> NSSTASKTYNYVYSSDPSSLNYLAENRAATSDIVANLVDGLLENDQYGNIIPSLAEDWTVSQDGLTYTYKLRKDAKWFTSEGEEYAPVTAQDFVTGLQYAADKKSEALYLVQDSVAGLDDYITGKTSDFSTVGVKALDDQTVQYTLVKPELYWNSKTLATILFPVNADFLKSKGDDFGKADPSSILYNGPFLMKALVSKSAIEYKKNPNYWDAKNVFVDDVKLTYYDGSDQESLERNFTAGAYTTARLFPNSSSYEGIKEKYKNNIIYSMQNSTSYFFNFNLDRKSYNYTSKTSDIEKKSTQEAVLNKNFRQAINFAFDRTSYGAQSEGKEGATKILRNLVVPPNFVSIKGKDFGEVVASKMVNYGKEWQGINFADGQDPYYNPEKAKAKFAEAKKELEAKGVQFPIHLDKTVEVTDKVGIQGVSSIKQSIESVLGSDNVVIDIQQLTSDEFDSSGYFAQTAAQKDYDLYHGGWGPDYQDPSTYLDIFNTNSGGFLQNLGLEPGEANDKAKAVGLDVYTQMLEEANKEQDPAKRYEKYADIQAWLIDSSLVLPSVSRGGTPSLRRTVPFAAAYGLTGTKGVESYKYLKVQDKIVTTDEYAKAREKWLKEKEESNKKAQEELAKHVK

Given the auxotrophic nature of pneumococci for certain amino acids, the Ami ABC transporter system, orchestrating oligopeptide uptake, becomes indispensable in host compartments lacking amino acids. The system comprises five exposed Oligopeptide Binding Proteins (OBPs) and four proteins building the ABC transporter channel. Crucially, SBPs determine the specificity of their respective transport systems, thereby governing the range of molecules capable of entering the cell. The five lipoproteins exhibit pairwise sequence identity of ~52–60% and share a very similar overall folding.

The crystal structure of AliB (residues 28–652) was solved at 1.65 Å resolution, revealing a closed conformation despite the absence of pre-incubation with any peptide. During the modeling and refinement process, additional electron density at the AliB substrate-binding site became evident, likely originating from Escherichia coli peptides bound during the purification process. Thus, we modeled E. coli peptides (VMVKGPGPGREST and PIVGGHEGAGV) previously reported to bind AliB. Although the electron density map clearly outlined the backbone of a nonapeptide, the side-chain density exhibited ambiguity in places, suggesting the binding of a heterogeneous population of peptides. Given that the observed peptide lengths did not align with the reported E. coli peptides, an identification effort was undertaken through mass spectrometry (see below). (A) Cartoon representation of AliB structure (colored green) in complex with an unknown oligopeptide(s) from E. coli modeled as poly-Ala (depicted as yellow capped sticks). The three-dimensional structures of AmiA and AliB revealed the capture of oligopeptides during their expression and purification from E. coli. Surprisingly, our analysis identified a total of 356 distinct peptides bound to the AmiA protein and 393 peptides bound to AliB. AmiA predominantly recognized peptides consisting of 10–11 residues, while AliB favored 11–12 residues.N-[5-[4-(5-{[(2R,6S)-2,6-DIMETHYL-4-MORPHOLINYL]METHYL}-1,3-OXAZOL-2-YL)-1H-INDAZOL-6-YL]-2-(METHYLOXY)-3-PYRIDINYL]METHANESULFONAMIDE | C24 H28 N6 O5 S | 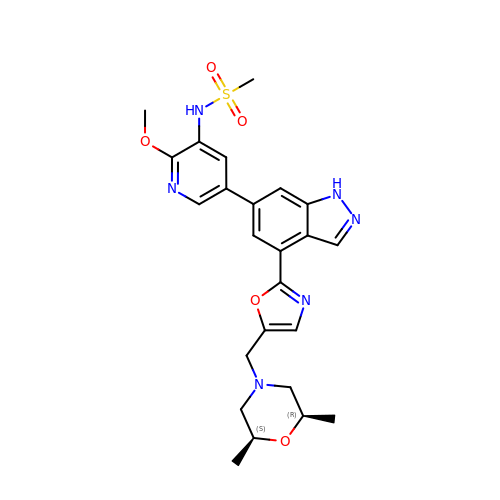NLUPPCTVKHDVIQ-GASCZTMLSA-N> MNHKVHMQYDIVAVTASAHDGNLPENTIDGNLSTRWSANGSGQYI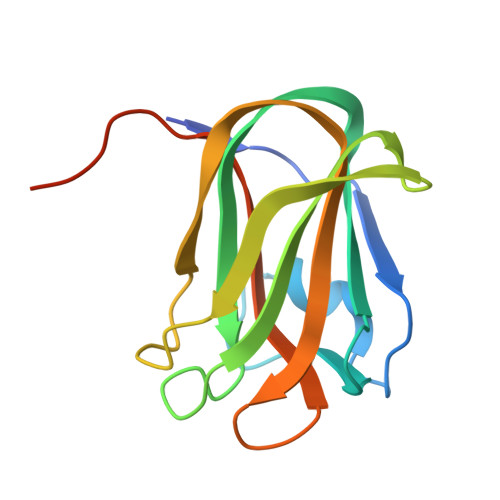TFDLGSAKTVNQVKAAWYNGDSRTSGFSISLGSDPASLTEVYSGTSSGQTNALESYSFTATTARYIRITGFGNSSNTWNSITEVAIFHAGEEGDGNEEHHHHHH> MNLDTLLPLQTIREHAKCDDNPRVTDDLLKLYREAAFEAAELYTGLSFTPEKTIVEPIRLKGRRGKIILSATPIAGRPVVFYGGGLGSPLELIPRPGSNVLFFPYGSPDRFQTWGDCHTCDVESQLMATYVTGRRCENSVPAGIIIGILKLIAWNINNPGDEVMSVRNTLNANA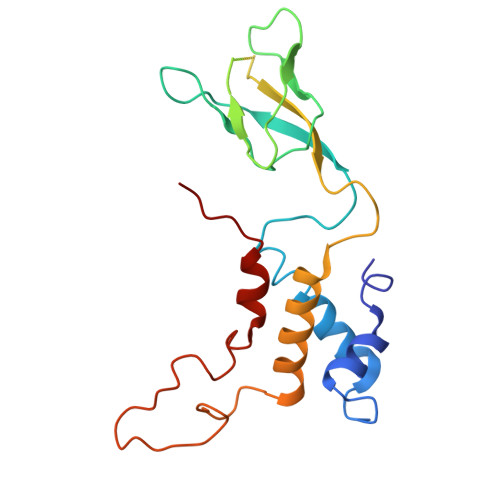QGLIGGTNNGAVISGAQDEWFRYRRVLL2-[(5S,10S)-11-[3,5-bis(oxidanyl)phenyl]-10-methyl-undecan-5-yl]-5-[(2S,7R)-7-fluoranyl-2-methyl-undecyl]benzene-1,3-diol | C36 H57 F O4 | 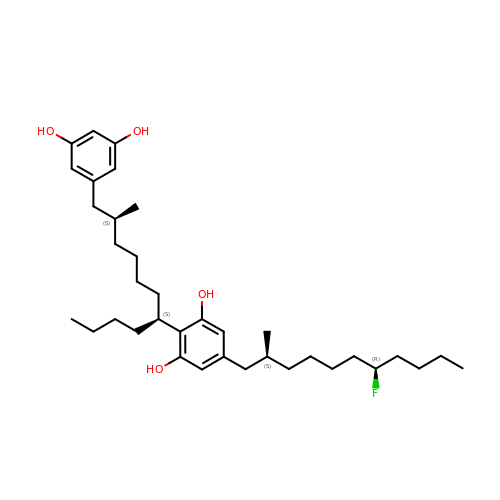FWCAPQCVEMEGNC-QQPIMWAISA-N Phenotype switching in Bacillus subtilis requires an all-or-none promoter binding of multiple ComK proteins. ComK target promoters consist of two elements (hereafter) separated by spacer sequences of variable length. Each box in a promoter contains an adenine–thymine (AT)-rich sequence. Cryo-EM structures of the complex between ComK and its promoter demonstrate that this coupling is due to mechanical forces that alter DNA curvature.

To assess the structural properties of the promoter, we engineered a set of comG promoters (18 bp spacer) that we site-specifically labelled with donor and acceptor fluorophores for confocal smFRET measurements. When we compared the experimental FRET efficiencies with theoretical values calculated for extended B-type DNA34, we noted substantial deviations across one box, suggesting an overall curved topology. Indeed, we obtained reduced FRET values that showed a better apparent agreement with the calculated B-DNA profile. This result indicated that the comG promoter is curved at neutral pH. To probe ComK binding cooperativity, we labelled the comG promoter with a FRET-pair either at each box or within the spacer. Fits with the Hill equation 38 result in Hill exponents of n = 3.6 ± 0.1 for box 1 and n = 3.4 ± 0.3 for box 2. To determine the precise arrangement of ComK on the DNA, we reconstructed the 3D maps of the complexes with spacers of 8 and 18 bp. The 3D maps show that ComK molecules in the two boxes face the same side of the DNA. In addition, we find a pseudo C2-symmetry of the protein density in each box, indicating two molecules of ComK per box, i.e., four per promoter, in excellent accord with the Hill exponents and a previous report. By contrast, we detected no ComK interactions across the spacer region, which suggests DNA-mediated allostery as source for the high binding cooperativity. In fact, the comG promoter contains an A-tract located 10 bp upstream of the first box 40 that is not occupied in our cryo-EM structure and controls indeed show that ComK is incapable of binding isolated A-tracts.

> CAGTTGAAAGTCTTTTTTCTTGCCAGAAAGAATTGGTTTTTCAGCATATAACATCTCACAAAATCACGTTTTCCCTGTTTGATTACCTTTTCT;> AGAAAAGGTAATCAAACAGGGAAAACGTGATTTTGTGAGATGTTATATGCTGAAAAACCAATTCTTTCTGGCAAGAAAAAAGACTTTCAACTG> MAGAIASRMSFSSLKRKQPKTFTVRIVTMDAEMEFNCEMKWKGKDLFDLVCRTLGLRETWFFGLQYTIKDTVAWLKMDKKVLDHDVSKEEPVTFHFLAKFYPENAEEELVQEITQHLFFLQVKKQILDEKIYCPPEASVLLASYAVQAKYGDYDPSVHKRGFLAQEELLPKRVINLYQMTPEMWEERITAWYAEHRGRARDEAEMEYLKIAQDLEMYGVNYFAIRNKKGTELLLGVDALGLHIYDPENRLTPKISFP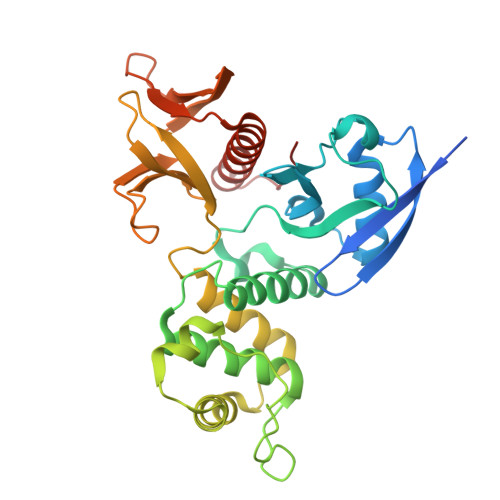WNEIRNISYSDKEFTIKPLDKKIDVFKFNSSKLRVNKLILQLCIGNHDLFMRRRKADSLEVQQ>[14x]MGKATTEEQKLIEDV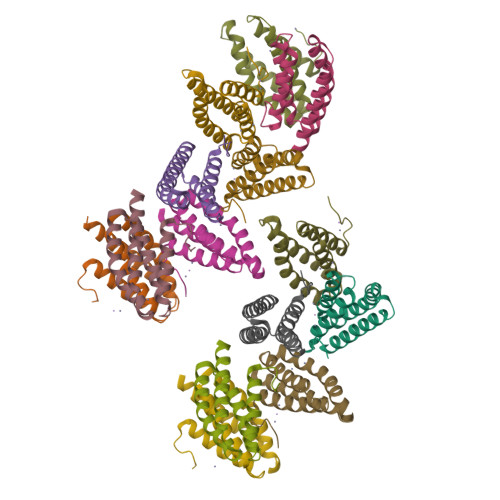NASFRAAMATTANVPPADKYKTFEAAFTVSSKRNLADAVSKAPQLVPKLDEVYNAAYNAADHAAPEDKYEAFVLHFSEALRIIAGTPEVHAVKPGA>SMRPPIVIHSSGKKYGFSLRAIRVYMGDSDVYTVHHVVWSVEDGSPAQEAGLRAGDLITHINGESVLG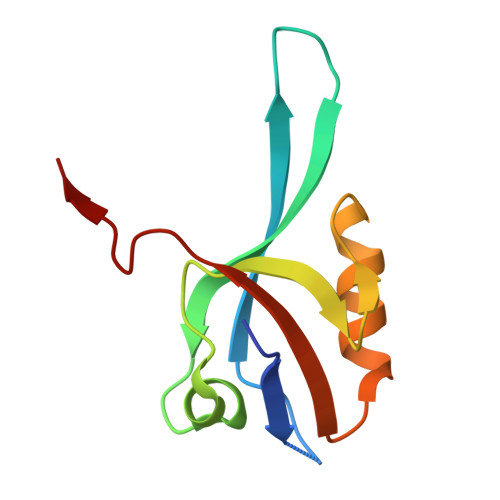LVHMDVVELLLKSGNKISLRTTALENTETSV[2x]> MKSSGAHGNVMGDAGVLKNEDESKYLDQVRYILKNGERIDDRTGTGTISVFGMHSVYSLRNGVVPVLTTKRVYWKGVVEELLWFIRGDTNAKHLSEKGVRIWDANGSRQFLDQCGFSDRSEGDLGPIYGFQWRHCGAEYRGMDTDYTNQGIDQLSEIIDLIKNEPHSRRIILSAWNVKDLKLMALPPCHTLAQFAVRNGELSCQ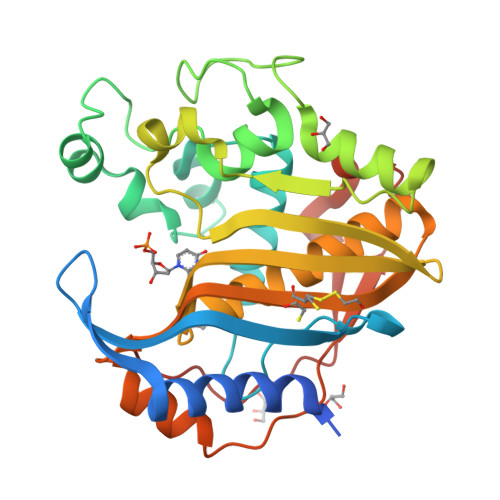LYQRSGDMGLGVPFNLASYGLLTHMIAHVCGLKTGHLCHVLGDAHVYMNHVDALQEQLKRQPRQFPTVRFIGNIKTIDDFTYESIVLENYQPMPAIKMAMAV> PAWDETN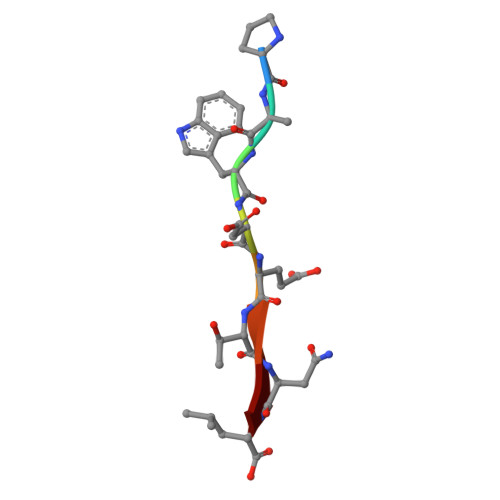L> MKHHHHHHHHGGLVPRGSHGGSEIKEGYFEQQQTLKNTATVNELSGIPAVDRAHVLQTALSIYPEVENWVAQFPVILPQRMGGMCLGMVATAPYAQPSVLVEASIMALIAFAIDDITEDVLSMTLTVEQIEAMLTLCVKLVQSGGNSTYRDYPELIQVFPTINESQPWVQLANALTKFCSEVQKFPAAAIYYSIFAKHFELYREAHCTELHWTQAVKEMGSYPTYEQYLLNSRKSIAAPLVESSLLAMVGEPVDSEFSLKPPYANLETLIDEVLLICGSSIRLANDIRSFEREPQAYQPNSLLILMLTQGCSQKEAEAILLKEIDTYLQKIETLISLLPSSLSTWGDS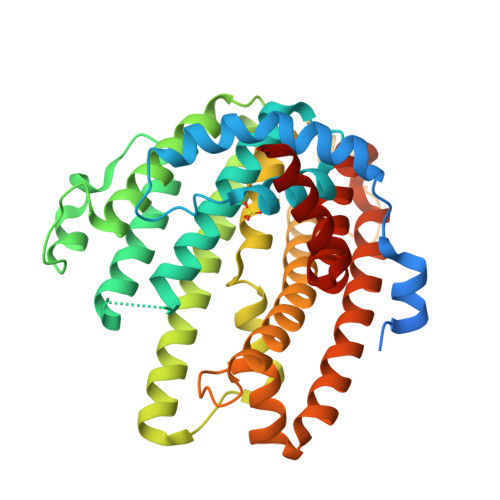ARRMSWFACTWYQTRDFHNFNKQMLAALR>GSHMGHWSQGLKISMQDPKMQVYKDEQVVVIKDKYPKARYHWLVLPWTSISSLKAVAREHLELLKHMHTVGEKVIVDFAGSSKLRFRLGYHAIPSMSHVHLHGISQDFDSPCLKNKKHWNSFNTEYFLESQAVIEMVQEAGRVTVRDGMPELLKLPLRCHECQQLLPSIPQLKEHLRKHWTQ[2x]

The APTX RNA‐DNA deadenylase protects genome integrity and corrects abortive DNA ligation arising during ribonucleotide excision repair and base excision DNA repair, and APTX human mutations cause the neurodegenerative disorder ataxia with oculomotor ataxia 1 (AOA1). The aprataxin (APTX) RNA/DNA polynucleotide deadenylase directly reverses 5′‐AMP damage (Ahel et al, 2006; Harris et al, 2009; Reynolds et al, 2009; Tumbale et al, 2011, 2014) and associates with DNA repair scaffolds XRCC1 (Cherry et al, 2015) and XRCC4. Environmental and metabolic sources of DNA damage prompt “abortive ligation”, the failure of ligase to complete step 3, and generation of 5′‐adenylated (5′‐AMP) DNA strand breaks (Ahel et al, 2006; Andres et al, 2015; Schellenberg et al, 2015). AOA1 mutations map to the APTX catalytic domain (Barbot et al, 2001; Moreira et al, 2001; Shimazaki et al, 2002; Le Ber et al, 2003; Tranchant et al, 2003; Criscuolo et al, 2004, 2005; Ito et al, 2005; Mosesso et al, 2005; Baba et al, 2007; Yokoseki et al, 2011) and cause variable age of disease onset.

For five amenable variants (V263G, H201Q, S242N, R199H, and L248M), we successfully crystallized and determined X‐ray structures of mutant proteins as ternary complexes with RNA‐DNA and AMP. V263G: Val263 maps to the β‐strand bearing the APTX catalytic nucleophile His260 and is a hydrophobic core residue engaging in Van der Waals interactions with neighboring Leu261 (β5), Val204 (β3), Ile232 (α2), His228 (α2), Phe246 (β4), and Val190 (β2). The structure of V263G (at 2.90 Å) reveals the mutation creates a sizeable cavity in the hydrophobic core corresponding to loss of the valine side chain. The structure of V263G shows the mutation creates a large cavity in the hydrophobic core, resulted from the loss of the valine side chain. Similar to core cavitation mutants of BRCA1 (Williams et al, 2003, 2004), V263G has severe impacts on stability and temperature‐dependent activity, being ~7‐fold more impaired for deadenylation activity at 37°C compared to 22°C.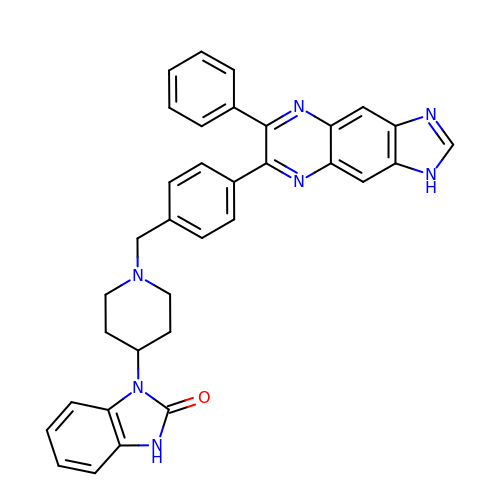1-(1-(4-(7-phenyl-1H-imidazo[4,5-g]quinoxalin-6-yl)benzyl)piperidin-4-yl)-1H-benzo[d]imidazol-2(3H)-one | C34 H29 N7 O | BIWGYFZAEWGBAL-UHFFFAOYSA-N>[4x]CCA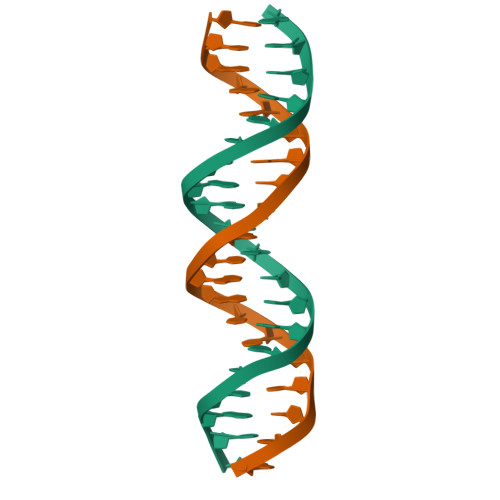ATAATCGCGATTATTGG>AQNNPYLFRSNKFLTLFKNQHGSLRLLQRFNEDTEKLENLRDYRVLEYCSKPNTLLLPHHSDSDLLVLVLEGQAILVLVNPDGRDTYKLDQGDAIKIQAGTPFYLINPDNNQNLRILKFAITFRRPGTVEDFFLSSTKRLPSYLSAFSKNFLEASYDSPYDEIEQTLLQEEQEGVIVKMPK[3x];>TLSSQDKPFNLRSRDPIYSNNYGKLYEITPEKNSQLRDLDILLNCLQMNEGALFVPHYNSRATVILVANEGRAEVELVGLEQQQQQGLESMQLRRYAATLSEGDIIVIPSSFPVALKAASDLNMVGIGVNAENNERNFLAGHKENVIRQIPRQVSDLTFPGSGEEVEELLENQKE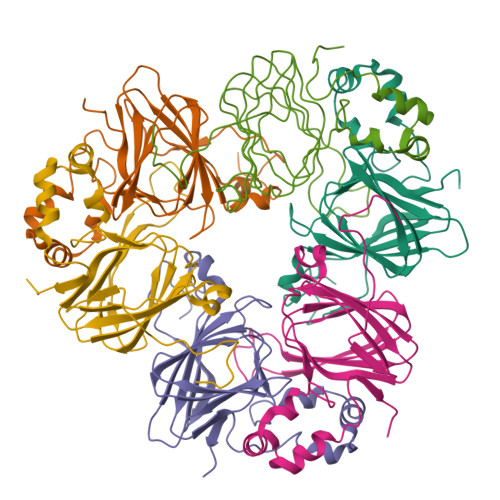SYFVDGQPR[3x]>[4x]MTEDNIAPITSVKVVTDKCTYKDNELLTKYSYENAVVTKTASGRFDVTPTVQDYVFKLDLKKPEKLGIMLIGLGGNNGSTLVASVLANKHNVEFQTKEGVKQPNYFGSMTQCSTLKLGIDAEGNDVYAPFNSLLPMVSPNDFVVS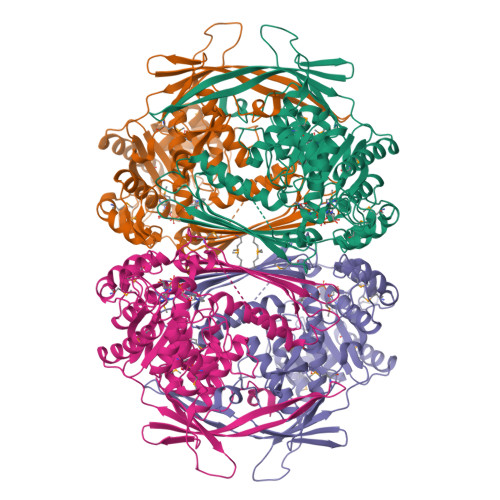GWDINNADLYEAMQRSQVLEYDLQQRLKAKMSLVKPLPSIYYPDFIAANQDERANNCINLDEKGNVTTRGKWTHLQRIRRDIQNFKEENALDKVIVLWTANTERYVEVSPGVNDTMENLLQSIKNDHEEIAPSTIFAAASILEGVPYINGSPQNTFVPGLVQLAEHEGTFIAGDDLKSGQTKLKSVLAQFLVDAGIKPVSIASYNHLGNNDGYNLSAPKQFRSKEISKSSVIDDIIASNDILYNDKLGKKVDHCIVIKYMKPVGDSKVAMDEYYSELMLGGHNRISIHNVCEDSLLATPLIIDLLVMTEFCTRVSYKKVDPVKEDAGKFENFYPVLTFLSYWLKAPLTRPGFHPVNGLNKQRTALENFLRLLIGLPSQNELRFEERLL>APVWGCASTRGRSAEMEDASAAVPRFADVPVRLLASRRDLDALGLDADALRLPAHLFGVFDGHGGAEVANYCRERIHVVLSAALARLGKNLGEMGEVDMKEHWDDVFTKCFQRVDDEVSGRVTRVVNGGGEVRSEPVTAENVGSTAVVALVCSSHVVVANCGDSRIVLCRGKEPVALSIDHKPDRKDERARIEAQGGKVIQWNGYRVLGVLAMSRSIGDRYLKPFVIPKPEVMVVPRAKDDDCLILASDGLWDVVSNEEACKVARRQILLWHKNNGAASPLSDEGEGSTDPAAQAAADYLMRLALKKGSEDNITVIVVDLKPRKKLKN[2x];>[2x]ETEYVRRFHRHEPRDHQCSSAVAKHIKAPVHLVWS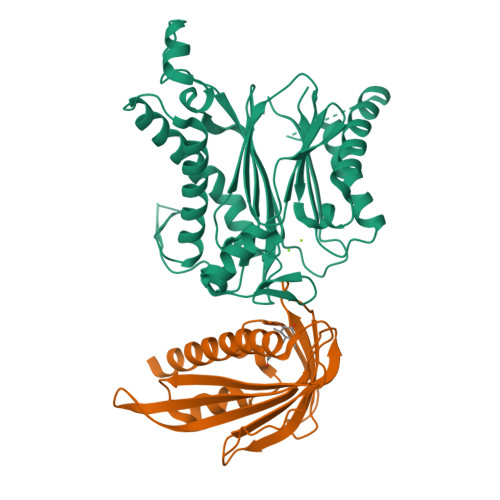LVRRFDQPQLFKPFVSRCEMKGNIEIGSVREVNVKSGLPATRSTERLELLDDNEHILSVRFVGGDHRLKNYSSILTVHPEVIDGRPGTLVIESFVVDVPEGNTKDETCYFVEALLKCNLKSLAEVSERLVVKDQTEPLDR>QDINAQLTTWFSQRLAGFSDEVVVTLRSSPNLLPSCEQPAFSMTGSAKLWGNVNVVARCANEKRYLQVNVQATGNYVAVAAPIARGGKLTPANVTLKRGRLDQLPPRTVLDIRQIQDAVSLRDLAPGQPVQLTMIRQAWRVKAGQRVQVIANGEGFSVNAEGQAMNNAAVAQNARVRMTSGQIVSGTVDSDGNILINLDPNSSSVDKLAAALEHHHHHH[2x]

FlgA is a periplasmic flagellar protein that chaperones P-ring formation. FlgA possesses a typical signal sequence at its N-terminus, recognized by the Sec-dependent pathway, suggesting that FlgA functions as a P-ring assembly chaperone in the periplasm. P-ring formation is a key step enabling the bacterial flagellum to pass through the outer membrane. FlgA can be divided into three domains, denominated as D1 (residues 1–74), D2 (residues 75–142), and D3 (residues 143–198).

The conformation of FlgA is different in the two forms. In the closed form, D3 is closer to D1 and forms a compact structure. This occurs largely because of a bend of about 70° around the Cα atom of R136. By studying the 3D structures of FlgA, we identified a pair of residues, R113 and S190, which are within a suitable distance for cross-linking with a disulfide bond that keeps the structure of FlgA in the closed conformation. To understand how the conformational difference between the open and closed forms of FlgA is related to its function, a disulfide bond was engineered by replacing these residues with cysteines (R113C and S190C, respectively). The disulfide bond forces FlgA to stay in the closed form and constrains the movement of domain D3. A rivet structure, which lacks the LP-ring of the hook basal-body, was isolated from the wild-type strain expressing FlgAR113C-S190C. These results indicate that the closed form of FlgA can bind to FlgI, but cannot proceed with subsequent steps, thereby inhibiting FlgI from forming the P-ring. The closed form of FlgA is reminiscent of the PapD structure, an immunoglobulin-like periplasmic chaperone for P pilus biogenesis. In the PapD structure, a deep cleft between domains constitutes the substrate recognition site; however, the cleft between FlgA domains D1 and D3 in the closed form might not be suitable for FlgI binding because the C-terminal domains of both forms of FlgA showed similar affinity for FlgI binding. Upon binding to FlgI, FlgA may adopt the closed structure, since FlgAR113C-S190C showed a strong negative dominant effect on motility of the wild-type strain.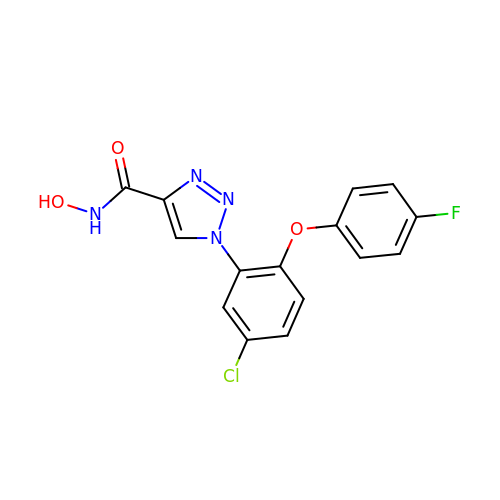1-[5-chloranyl-2-(4-fluoranylphenoxy)phenyl]-~{N}-oxidanyl-1,2,3-triazole-4-carboxamide | C15 H10 Cl F N4 O3 | NXLUFTCWMNFMML-UHFFFAOYSA-N2-(2-methyl-5-nitro-1H-imidazol-1-yl)ethyl [(1R)-2,2,2-trichloro-1-(pyrimidin-2-ylamino)ethyl]carbamate | 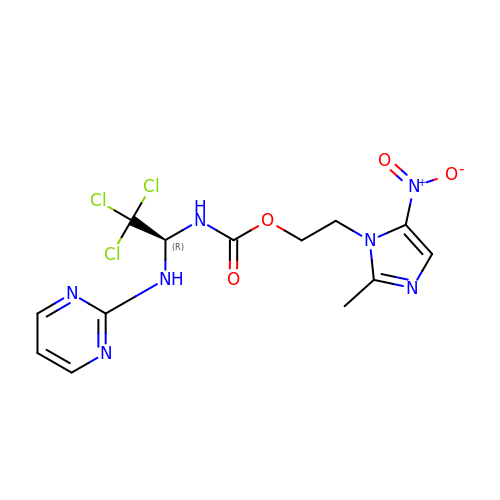C13 H14 Cl3 N7 O4 | ZEXHXVOGJFGTRX-SNVBAGLBSA-N>[4x]M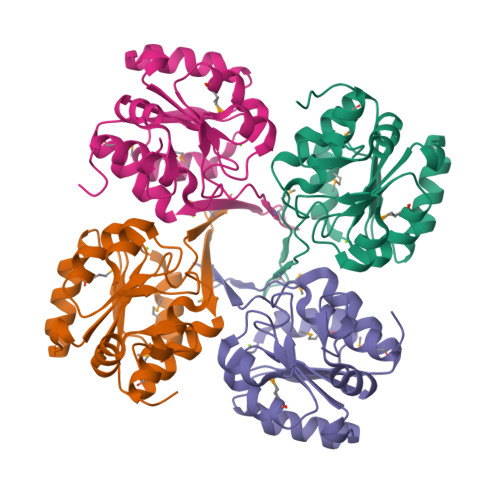SLSSTVSTLYGEVEPSLLEIAKQIKLLICDVDGVFSDGLIYMGNQGEELKTFHTRDGYGVKALMNAGIEIAIITGRRSQIVENRMKALGISLIYQGQDDKVQAYYDICQKLAIAPEQTGYIGDDLIDWPVMEKVALRVCVADGHPLLAQRANYVTHIKGGHGAVREVCDLILQARNELDVHKGLSLEGHHHHHH>EETPVTPQPPDILLGPLFNDVQNAKLFPDQKTFADAVPNSDPLMILADYRMQQNQSGFDLRHFVNVNFTLPKEGEKYVPPEGQSLREHI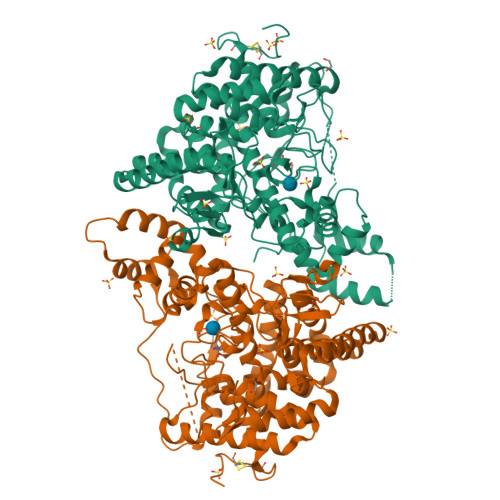DGLWPVLTRSTENTEKWDSLLPLPEPYVVPGGRFREVYYWDSYFTMLGLAESGHWDKVADMVANFAHEIDTYGHIPNGNRSYYLSRSQPPFFALMVELLAQHEGDAALKQYLPQMQKEYAYWMDGVENLQAGQQEKRVVKLQDGTLLNRYWDDRDTPRPESWVEDIATAKSNPNRPATEIYRDLRSAAASGWDFSSRWMDNPQQLNTLRTTSIVPVDLNSLMFKMEKILARASKAAGDNAMANQYETLANARQKGIEKYLWNDQQGWYADYDLKSHKVRNQLTAAALFPLYVNAAAKDRANKMATATKTHLLQPGGLNTTSVKSGQQWDAPNGWAPLQWVATEGLQNYGQKEVAMDISWHFLTNVQHTYDREKKLVEKYDVSTTGTGGGGGEYPLQDGFGWTNGVTLKMLDLICPKEQPCDNVPATRPTVKSATTQPSTKEAQPTP[4x]>TTPSMEDYIKQIYMLIEEKGYARVSDIAEALAVHPSSVTKMVQKLDKDEYLIYEKYRGLVLTSKGKKIGKRLVYRHELLEQFLRIIGVDEEKIYNDVEGIEHHLSWNS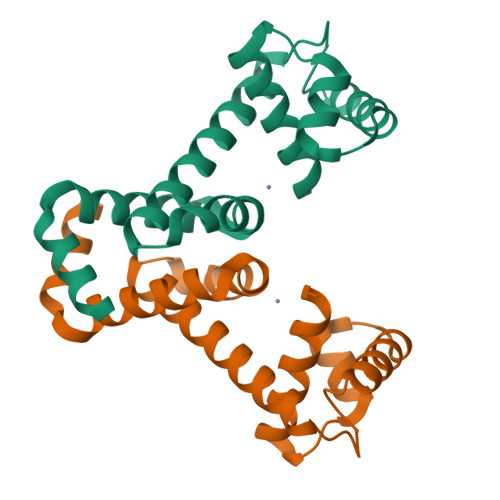IDRIGDLVQYFEEDDARKKDLKSIQKKTEHHNQ[2x]The sulfonamides (sulfas) are the oldest class of antibacterial drugs and inhibit the bacterial dihydropteroate synthase (DHPS, encoded by folP), through chemical mimicry of its co-substrate p-aminobenzoic acid (pABA). Resistance to sulfa drugs is mediated either by mutations in folP or acquisition of sul genes, which code for sulfa-insensitive, divergent DHPS enzymes. DHPS catalyzes the condensation of para-aminobenzoic acid (pABA) and 6-hydroxymethyl-7,8-dihydropterin pyrophosphate (DHPP), producing 7,8-dihydropteroic acid (7,8-DHP); this compound is further transformed, ultimately leading to tetrahydrofolate, an essential precursor for DNA and RNA synthesis. All three Sul enzymes adopted the (ɑ/β)8 TIM barrel fold also shared by DHPS.

We determined the crystal structure of Sul1 in a ligand-bound state, and the Sul2 and Sul3 enzymes in both apo and ligand-bound forms to resolutions between 1.74 to 2.8 Å. Comparison of Sul apo and ligand-bound structures revealed conformational changes in these three loops triggered by ligand binding. In particular, loop 1 is oriented further away from the ligand-binding cleft in the apo structures of Sul2 and Sul3 as compared to the structures of these enzymes in 7,8-DHP or pABA-bound states. Similarly, loop 3 in Sul2 and Sul3 also undergoes a large conformational change upon binding of pABA or 7,8-DHP. Finally, in the Sul2 and Sul3 structures, loop 2 undergoes conformational changes in a more confined space in presence of the ligands. We noticed that the Phe residue that is conserved across Sul enzymes (Phe178 in Sul1, Phe179 in Sul2 and Phe177 in Sul3) and localized to the active site adopted different rotamer conformations depending on ligand binding. In general, the sidechain of this residue and its environment (ɑ6) showed higher crystallographic B-factors than the average protein (i.e., for the Sul2 apo structure, B-factor of Phe179 sidechain atoms were 32 to 67, for ɑ6: 20 to 53, and for the protein average: 36).

>[4x]MNKSLIIFGIVNITSDSFSDGGRYLAPDAAIAQARKLMAEGADVIDLGPASSNPDAAPVSSDTEIARIAPVLDALKADGIPVSLDSYQPATQAYALSRGVAYLNDIRGFPDAAFYPQLAKSSAKLVVMHSVQDGQADRREAPAGDIMDHIAAFFDARIAALTGAGIKRNRLVLDPGMGFFLGAAPETSLSVLARFDELRLRFDLPVLLSVSRKSFLRALTGRGPGDVGAATLAAELAAAAGGADFIRTHEPRPLRDGLAVLAALKETARIR>GPLGSWPAVTGDSPHLTNFGRKLLKDCRQVQKPIGGYENLGNVIKLSAEFPLEFGVNSVKVYRQSPSRLARINEEVASAYPLIHERTLGLYLQYLEHKCRWGNAVEKPIYRNLSLCGFVQRLLVKRCASFFARNDKYLLVSGESGASGFEAVGTREEKAPLVLANVLSYDDIKLSALLSVSSRTEFVNEGERTNCGHVDLNTKTLERHGVIVGMIGARLSRRNLMEFQDIVIARQQNTRERGYGMALDEPATTRDEDYRRLWREFYATRDLIHGQAVIDNQRFGPSKNKMDVFDNLVMKRRYAISFDML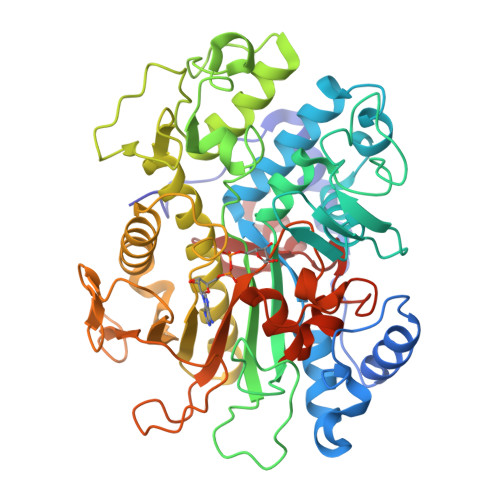LLEAEARAKRVKKLAYIHVVGFGLGVWKAAEQQERIFMETFEQRMRTLGNRLNNVGLVHFSWFSITHCGGLSNGSLIEIPGHPKDGIRVLISKRNPARKLSDPEHAGMLLVVSYAWDGNALPGNEFWMKMLQSTGDSSTACSTLVAELHNPYINTKFCNGGNLHIASPEHGVLHIAEYAKRVI[4x]>MNIILKISGKFFDEDNVDNLIVLRQSIKELADNGFRVGIVTGGGSTARRYIKLAREIGIGEAYLDLLGIWASRLNAYLVMFSLQDLAYMHVPQSLEEFIQDWSHGKVVVTGGFQPGQSTAAVAALVAEASSSKTLVVATNVDGVYEKDPRIYADVKLIPHLTTQDLRKILEGSQSVQAGTYELLDPLAIKIVERSKIRVIVMNYRKLNRIIDILKGE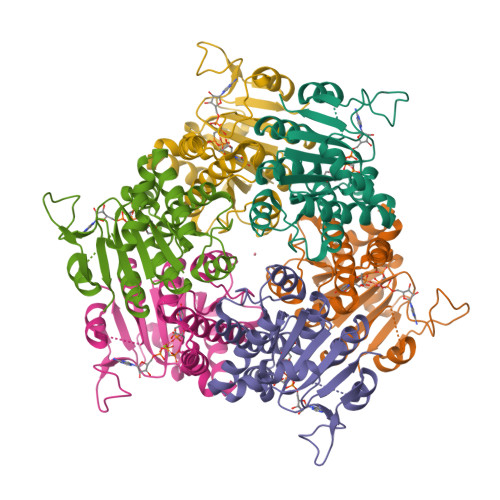EVSSIIEPV[6x]>[2x]VVVVNKQVLLKHFIPEGAPKETDMELVTTGTIRLRVPEGSNAVLLKNLYLSCDPYMRMRMTKHEEASYVDDFVPGAPITGFGVGKVVDSSHPDFKTGDYVWGLIGWE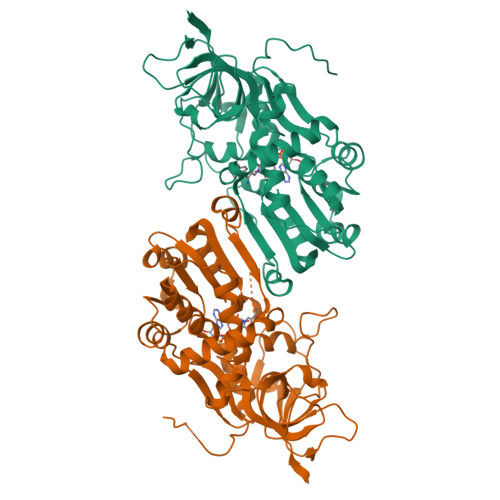EYSLITKPQGLFKIHHTEIPLSYYTGILGMVGLTAYVGFYDICSPKKGERVFVSAAAGAVGQIVGQFAKQFGCYVVGSAGSDEKVNLLKTKFGFDEAFNYKKEPDLTKALKRYFPEGIDIYFENVGGPMLEAVLHNMRIKGRIAACGMISQYNLEKPEGVHNLFLIVGKRIRLEGFLVFDHYGSYPEFEEKVVQLIKEEKIKYLEDIVEGLENAPAALIGLFEGRNVGKQVVVVSREKGHHHHHH> MKTEWPELVGKSVEEAKKVILQDKPEAQIIVLPVGTIVTMEYRIDRVRIFVDKLDNIAQVPRVG

CI2 is a small single domain protein of 64 residues, which has been extensively used as a model to understand key concepts of protein folding and stability. L49 and I57 are both part of the folding nucleus in CI2 and very important for the stability of the folded state of CI232. Here, we have applied an efficient in-cell assay in E. coli to select variants of the barley chymotrypsin inhibitor 2 with increased stability. We, therefore, determined the crystal structures of all four CI2 variants in the wild-type to L49I/I57V double mutant cycle.

In contrast, introducing L49I, which on its own destabilizes by ΔΔGf = 3.4 ± 0.1 kJ mol−1, together with I57V results in a total stabilization of the L49I/I57V double mutant of ΔΔGf = −3.8 ± 0.1 kJ mol−1. Overall, the structures of L49I, I57V and L49I/I57V are highly similar to the structure of the wild-type with RMSDs for the backbone of 0.16, 0.45 and 0.17 Å. The Ile at position 49 in L49I is oriented similarly to the Leu in wild-type and I57V. The Val at position 57 in I57V and L49I/I57V superimpose, except for the missing δ1 methyl group, with the Ile at position 57 in the wild-type and L49I. Analysis of the pairwise interaction energies at the residue level suggests that much of the stabilizing effect of the I57V mutation originates from an unfavourable interaction between I57 and Q59 that is observed in structures of both the wild-type and L49I. The effect of the L49I mutation, which destabilizes the wild-type, but stabilizes the I57V variant is more subtle and not easily explained from the crystal structures. It appears that some of the destabilization of the L49I mutation is a long-range effect resulting in several less favourable interactions among residues 57-62. These negative effects are relieved in the double mutant.1-(4-{3,5-dichloro-4-[(2,4-dimethylpyridin-3-yl)methoxy]phenyl}pyridin-2-yl)piperazine 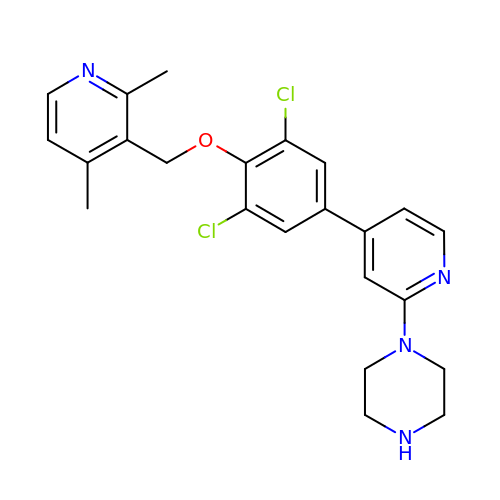| C23 H24 Cl2 N4 O | UBIXTVHUCALUIC-UHFFFAOYSA-N> DSLRPKLSEEQQRIIAILLDAHHKTYDPTYSDFCQFRPPVRVNDGGGSVTLELSQLSMLPHLADLVSYSIQKVIGFAKMIPGFRDLTSEDQIVLLKSSAIEVIMLRSNESFTMDDMSWTCGNQDYKYRVSDVTKAGHSLELIEPLI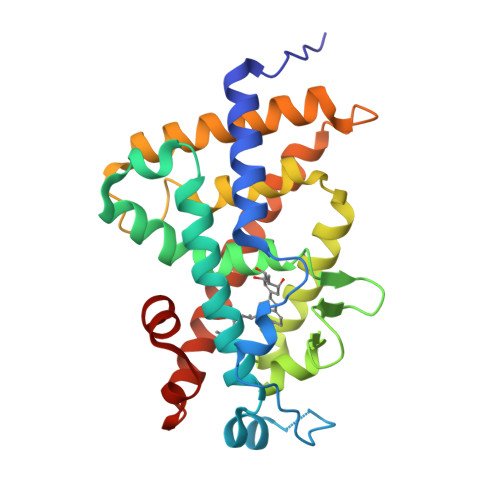KFQVGLKKLNLHEEEHVLLMAICIVSPDRPGVQDAALIEAIQDRLSNTLQTYIRCRHPPPGSHLLYAKMIQKLADLRSLNEEHSKQYRCLSFQPECSMKLTPLVLEVFG Here, we use biochemical, biophysical and structural analyses to show how a bacteriocin exploits TolC, a major outer-membrane antibiotic efflux channel in Gram-negative bacteria, to transport itself across the outer membrane of target cells. Klebicin C (KlebC), a rRNase toxin produced by Klebsiella pneumoniae, binds TolC of a related species (K. quasipneumoniae) with high affinity through an N-terminal, elongated helical hairpin domain common amongst bacteriocins. TolC is one of the most prevalent drug efflux channels in bacteria and is frequently associated with multidrug resistance. Our results indicate that TolC, in addition to its known role in antibiotic export, can function as a protein import channel for bacteriocins.

K. quasipneumoniae Qmp M1-977 is a KlebC susceptible strain in which TolC (KqTolC) shares 83% sequence identity with E. coli K-12 TolC. KqTolC was expressed and purified for single-particle cryo-EM studies to resolve the structure of the KqTolC-KlebC1-254 complex. KqTolC is a 150-kDa homotrimer comprised of 50-kDa subunits, each contributing four β-strands to form a single 12-stranded β-barrel across the outer membrane. The remainder of each subunit adopts a helical structure forming an elongated channel. Whilst the β-barrel in the membrane is exposed to the extracellular environment the α-helical segment of the protein forms an iris in the periplasm. The position of extracellular loops within the structure defines the accessible size of the β-barrel, creating a more open configuration in KqTolC relative to E. coli TolC. Although some local distortions are observed at the iris where helices meet, none significantly alter the effective diameter of the iris (4–5 Å at its narrowest point). We can discount the possibility that these sequences pass between the periplasmic helices of the TolC channel since the positions of the helices are essentially identical in the KlebC-bound and unliganded forms of KqTolC.

>MKKLLPILIGLSLTGFSAMSQAENLLQVYQQARISNPDLRKSAADRDAAFEKINEARSPLLPQLGLGADYTYTSGFRDYKDQNSNVTSGSLQLTQVLFDMSKWRALTLQEKAAGIQDVTYQTDQQTLILNTATAYFKVLAAIDTLSYTEAQKQAIYRQLDQTTQRFNVGLVAITDVQNARSQYDAVLANEVTARNDLDNAVEELRQVTGNYYPELASLNVDGFKTSKPQAVNALLKEAENRNLSLLQARLNQDLAREQIRQAQDGHLPTLDLNASSGVSNNRYSGSKSISQDADIGQNKIGLSFSLPLYQGGMVNSQVKQAQYNFVGASEQLESAHRSVVQTVRSSFNNVNASISSINAYKQAVVSAQSSLDAMEAGYSVGTRTIVDVLDATTTLYNAKQQLSNARYNYLINELNIKSALGTLNEQDLIALNNTLGKPISTSADSVAPENPQQDATADGYGNTTAAMKPASARTTTHSSGSNPFRQLEHHHHHH[3x]>[2x]MFKTEFEFPEELKTKLQEHINYFPKKRQAILLCLHEIQNYYGYIPPESLKPLADMLELPLNHVEGVVAFYDMFDREDKAKYRIRVCVSIVCHLMGTNKLLKALENILGIKPGEVTPDGKFKIVPVQCLSACSEAPVFMVNDDEYKFESEVQLNEILSRYT;>MRSYPAIPRIYAETTLNMLLKRAKKPRVHSIDEYLKDGGYQALEKALNMSPEEIIDWVDKSTLRGRGGAGFPTGKKWKFAVQNPGPRYFICNADESEPGTFKDRIIIERDPHLLIEGII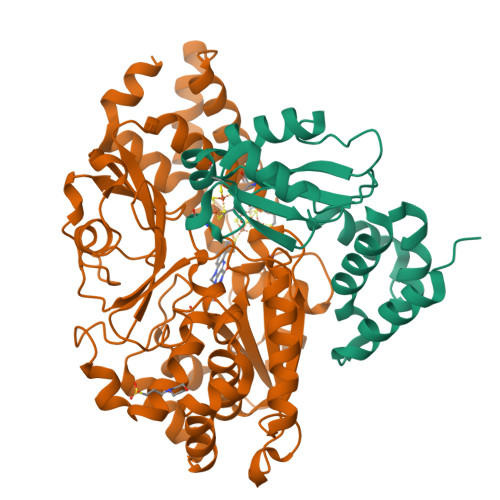ISSYAIGANEAYIYIRGEYPAGYYILRDAIEEAKKKGFLGKNILGSGFDLEIYVARGAGAYICGEETALIESLEGKRGHPRLKPPYPVQKGLWGKPTVVNNVETIANVPFIISMGWEEYRYIGPSDYAGPKLFPVSGKVKKPGVYELPMNTTLREVIFKYAGGTLGNKKVKAVFSGALDCFSSEELDIPMDYSPLGFGGTGTVIVLTEEDDIVEAALKIAEFYEHETCGQCTPCRVGCYEQANLLEKIYKGEATEQDWEGFDFVNRNIQPTSICGLGAVAGRLIRQTLEKFPEEWEKYRKKSASLPLAGHHHHHH[2x]>CCTTTAA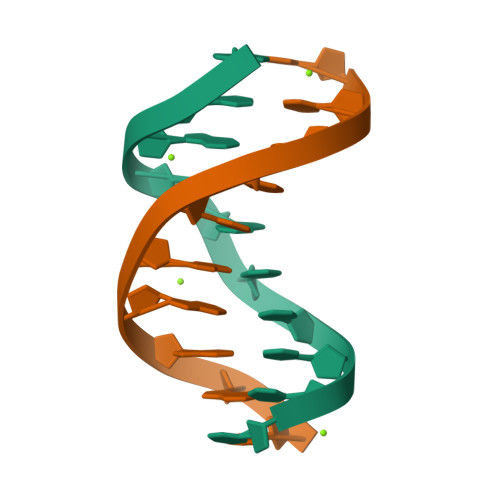AGG[2x]>[7x]MSIPVTEFRQFSEQQPAFRVLKPWWDVFTDYLSVAMLMIGVFGCTLQVMQDKIICLPKRVQPAQNHSSLSNVSQAVASTTPLPPPKPSPANPITVEMKGLKTDLDLQQYSFINQMCYERALHWYAKYFPYLVLIHTLVFMLCSNFWFKFPGSSSKIEHFISILGKCFD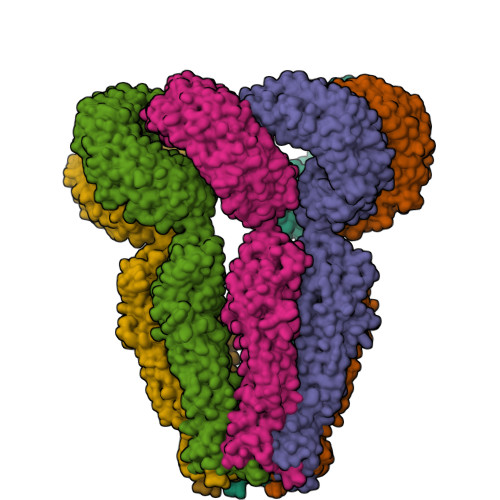SPWTTRALSEVSGEDSEEKDNRKNNMNRSNTIQSGPEGSLVNSQSLKSIPEKFVVDKSTAGALDKKEGEQAKALFEKVKKFRLHVEEGDILYAMYVRQTVLKVIKFLIIIAYNSALVSKVQFTVDCNVDIQDMTGYKNFSCNHTMAHLFSKLSFCYLCFVSIYGLTCLYTLYWLFYRSLREYSFEYVRQETGIDDIPDVKNDFAFMLHMIDQYDPLYSKRFAVFLSEVSENKLKQLNLNNEWTPDKLRQKLQTNAHNRLELPLIMLSGLPDTVFEITELQSLKLEIIKNVMIPATIAQLDNLQELSLHQCSVKIHSAALSFLKENLKVLSVKFDDMRELPPWMYGLRNLEELYLVGSLSHDISRNVTLESLRDLKSLKILSIKSNVSKIPQAVVDVSSHLQKMCIHNDGTKLVMLNNLKKMTNLTELELVHCDLERIPHAVFSLLSLQELDLKENNLKSIEEIVSFQHLRKLTVLKLWHNSITYIPEHIKKLTSLERLSFSHNKIEVLPSHLFLCNKIRYLDLSYNDIRFIPPEIGVLQSLQYFSITCNKVESLPDELYFCKKLKTLKIGKNSLSVLSPKIGNLLFLSYLDVKGNHFEILPPELGDCRALKRARLVVEDALFETLPSDVREQMKADALEVLFQ>[2x]RFLKVKNWETDVVLTDTLHLKSTLETGCTEHICMGSIMLPSQHTRKPEDVRTKDQLFPLAKEFLDQYYSSIKRFGSKAHMDRLEEVNKEIESTSTYQLKDTELIYGAKHAWRNASRCVGRIQWSKLQVFDARDCTTAHGMFNYICNHVKYATNKGNLRSAITIFPQRTDGKHDFRVWNSQLIRYAGYKQPDGSTLGDPANVQFTEICIQQGWKAPRGRFDVLPLLLQANGNDPEL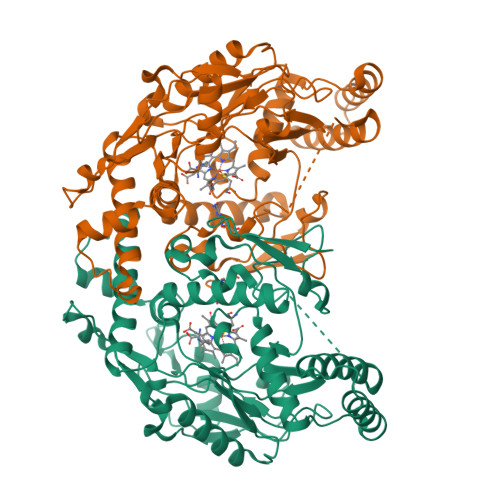FQIPPELVLEVPIRHPKFDWFKDLGLKWYGLPAVSNMLLEIGGLEFSACPFSGWYMGTEIGVRDYCDNSRYNILEEVAKKMDLDMRKTSSLWKDQALVEINIAVLYSFQSDKVTIVDHHSATESFIKHMENEYRCRGGCPADWVWIVPPMSGSITPVFHQEMLNYRLTPSFEYQPDPWNTHVWK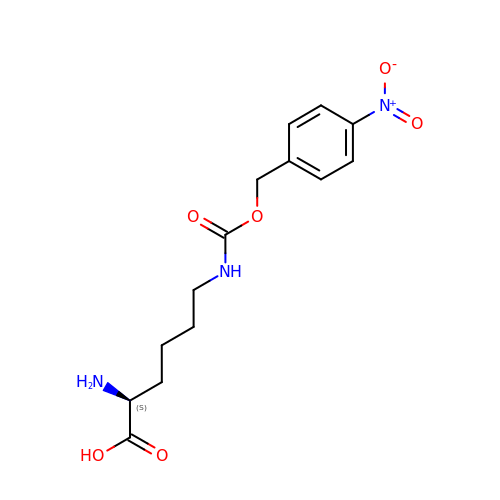N6-{[(4-nitrophenyl)methoxy]carbonyl}-L-lysine | C14 H19 N3 O6 | XMTCOKGMBIHVBJ-LBPRGKRZSA-N>GSHMRVQVSGLSDETTWHTLKDHLRQAGEVTFCKVFSGGRA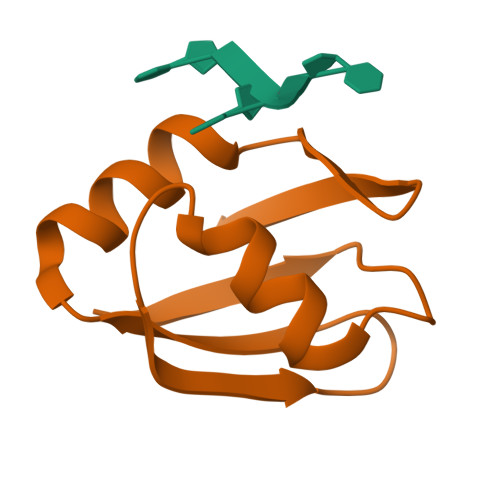VVEFVTPEDAARAITELQASELEGATLFLR[9x]>SLDIQSLDIQCEELSDARWAELLPLLQQCQVVRLDDCGLTEARCKDISSALRVNPALAELNLRSNELGDVGVHCVLQGLQTPSCKIQKLSLQNCCLTGAGCGVLSSTLRTLPTLQELHLSDNLLGDAGLQLLCEGLLDPQCRLEKLQLEYCSLSAASCEPLASVLRAKPDFKELTVSNNDINEAGVRVLCQGLKDSPCQLEALKLESCGVTSDNCRDLCGIVASKASLRELALGSNKLGDVGMAELCPGLLHPSSRLRTLWIWECGITAKGCGDLCRVLRAKESLKELSLAGNELGDEGARLLCETLLEPGCQLESLWVKSCSFTAACCSHFSSVLAQNRFLLELQISNNRLEDAGVRELCQGLGQPGSVLRVLWLADCDVSDS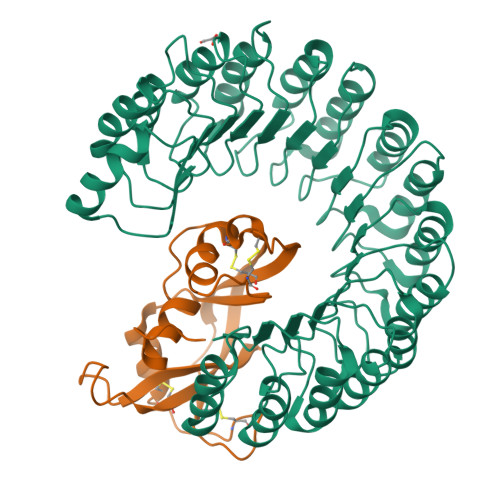SCSSLAATLLANHSLRELDLSNNCLGDAGILQLVESVRQPGCLLEQLVLYDIYWSEEMEDRLQALEKDKPSLRVIS[2x];>[2x]MKPPQFTWAQWFETQHINMTSQQCTNAMQVINNYQRRCKNQNTFLLTTFANVVNVCGNPNMTCPSNKTRKNCHHSGSQVPLIHCNLTTPSPQNISNCRYAQTPANMFYIVACDNRDQRRDPPQYPVVPVHLDRII> AHKNRIFVSSSKDFEGYPSKAIVPVQFVALLTSIHLTETKCLLGFSNFERRGDQSQEDQYLIKLKFKDRGSERLARITISLLCQYFDIELPDLDSDSGASPTVILRDIHLERLCFSSCKALYVSKHGNYTLFLEDIKPLDLVSVISTISTKS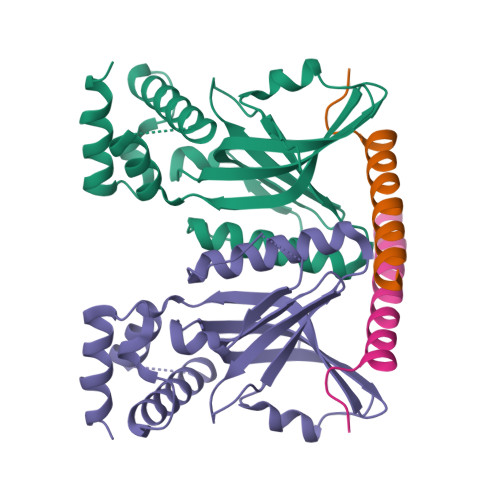TNSSKHSSSELISECDLNNSLVDIFNNLIEMNRDEKNRFKFVKLIHYDIELKKFVQDQQKVLSQKSKAAAINPFFVPNRLG;> SPLKLQSRKLRYANDVQDLLDDVENSPVVATKRQNV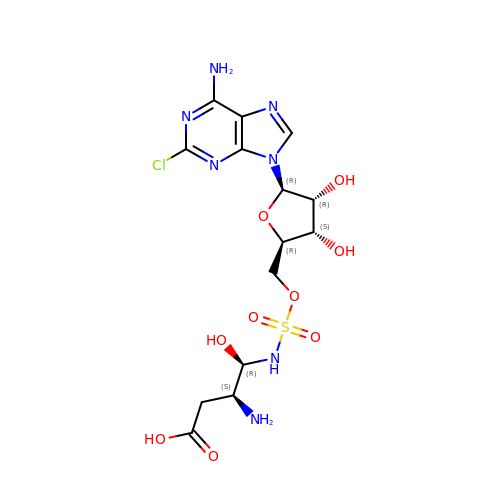9-(5-O-{[(1R,2R)-2-amino-3-carboxy-1-hydroxypropyl]sulfamoyl}-beta-D-lyxofuranosyl)-2-chloro-9H-purin-6-amine | C14 H20 Cl N7 O9 S | YOQULUZFJUCTJA-UHFFFAOYSA-N5-[(3S)-3-methoxy-3-(3,4,5-trimethoxyphenyl)prop-1-yn-1-yl]-6-methylpyrimidine-2,4-diamine 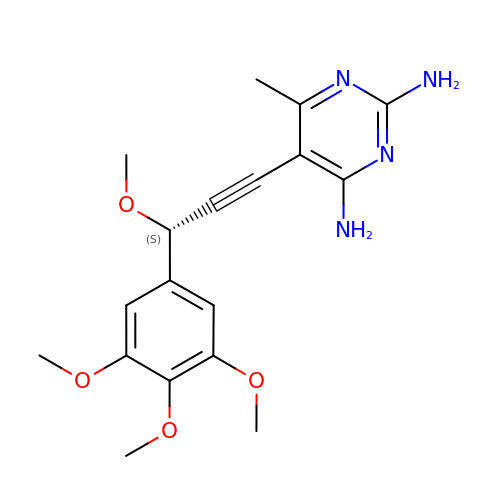| C18 H22 N4 O4 | WGUCJULKGMTPOP-CYBMUJFWSA-N> RQANELPGAPSQEEAVIAFGKFKLNLGTREMFREDEPMPLTSGEFAVLKALVSHPREPLSRDKLMNL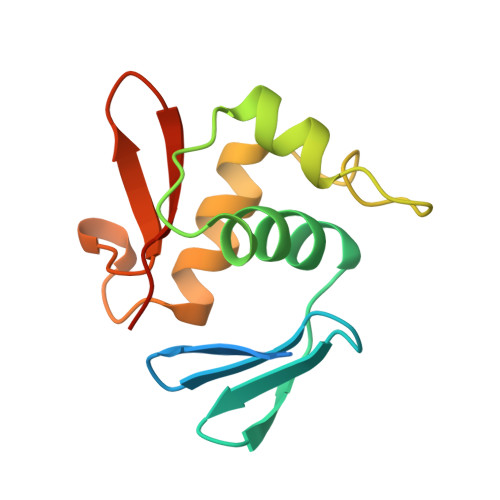ARGREYSAMERSIDVQISRLRRMVEEDPAHPRYIQTVWGLGYVFVPDGSKA>GHMSTLLINQPQYAWLKELGLREENEGVYNGSWGGRGEVITTYCPANNEPIARVRQASVADYEETVKKAREAWKIWADIPAPKRGEIVRQIGDALREKIQVLGSLVSLEMGKILVEGVGEVQEYVDICDYAVGLSRMIGGPILPSERSGHALIEQWNPVGLVGIITAFSFPVAVYGWNNAIAMICGNVCLWKGAPTTSLISVAVTKIIAKVLEDNKLPGAICSLTCGGADIGTAMAKDERVNLLSFTGSTQVGKQVGLMVQERFGRSLLELGGNNAIIAFEDADLSLVVPSALFAAVGTAGQRCTTARRLFIHESIHDEVVNRLKKAYAQIRVGNPWDPNVLYGPLHTKQAVSMFLGAVEEAKKEGGTVVYGG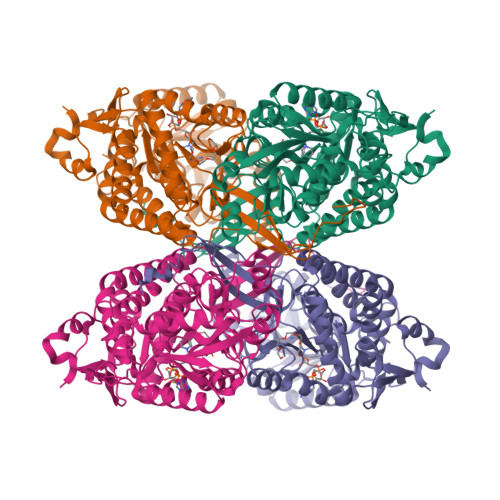KVMDRPGNYVEPTIVTGLGHDASIAHTETFAPILYVFKFKNEEEVFAWNNEVKQGLSSSIFTKDLGRIFRWLGPKGSDCGIVNVNIPTSGAEIGGAFGGEKHTGGGRESGSDAWKQYMRRSTCTINYSKDLPLAQGIKFQ[8x]>GMAALLSQRQKRYQQFLAMKMTQVFDILFSLTRGQPYTETYLSSLIVDSLQDSNNPIGTKEASEILAGLQGILPMDISVHQVDGGLKVYRWNSLDKNRFSKLLQIHKSKQQD[2x]

The process of eukaryotic DNA replication begins during G1 phase with the loading of the minichromosome maintenance (MCM) heterohexamer comprising Mcm2–7 subunits into head-to-head double hexamers with double-stranded DNA passing through the length of a long central channel. This topological loading requires the Origin Recognition Complex (ORC), Cdc6 and Cdt1 proteins. In budding yeast, Cdt1 forms a stable complex with MCM before loading. We propose that Cdt1 stabilizes a conformation of the MCM ring in which the Mcm2–5 gate is held open to allow duplex DNA passage required for helicase loading. To understand Cdt1–MCM at an atomic level, we determined crystal structures of two non-overlapping fragments of S. cerevisiae Cdt1 spanning amino acid residues 1–438 and 495–604.

The structure of Cdt1(495–604) revealed the C domain, which is highly similar to the analogous WHD domain previously characterized in mouse Cdt1. Further division of the C terminus of Cdt1 showed that fragments containing amino acid residues 271–496 and 495–604 interacted with both Mcm2 and 6, suggesting there are multiple interactions between Cdt1 and MCM subunits. Although the C-terminal WHD of Cdt1 could be accommodated in our EM structure, interacting with the WHD of Mcm6, we have not modelled this region using our negative stain data, due to the limited resolution. Our CTD-Cdt1 crystal structure can however be docked into the 7 Å resolution cryo-EM structure of MCM-Cdt1, indicating that the C-terminal WHD of Cdt1 interdigitates between the A domains of Mcm4 and Mcm6, in agreement with two recently published atomic models.> GSSTEGTERVRPQRVEQKLPPLSWGGSGVQTAYWVQEAVQPGDSLADVLARSGMARDEIARITEKYGGEADLRHLRADQSVHVLVGGDGSAREVQFFTDEDGERNLVALEKKGGIWRRSASDADMKVLPTLRSVVVKTSARGSLARAEVPVEIRESLSGIFAGRFSLDGLKEGDAVRLLYDSLYFHGQQVAAGDILAAEVVKGGTTHQAFYYRSDKEGGGGGNYYDEDGRVLQEKGGFNIEPLVYTRISSPFGYRMHPILHTWRLHTGIDYAAPQGTPVRASADGVITFKGRKGGYGNAVMIRHANGVETLYAHLSAFSQAQGNVRGGEVIGFVGSTGRSTGPHLHYEARINGQPVNPVSVA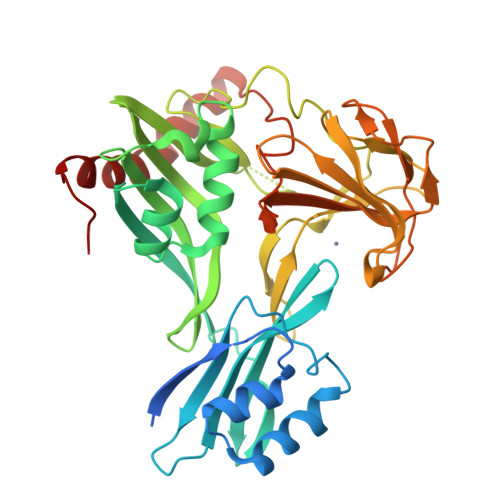LPTPELTQADKAAFAAQKQKADALLARLRGIPVTVSQSD> ALPQTVRIGTDTTYAPFSSKDAKGEFIGFAIDLGNEMCKRMQVKCTWVASDFDALIPSLKAKK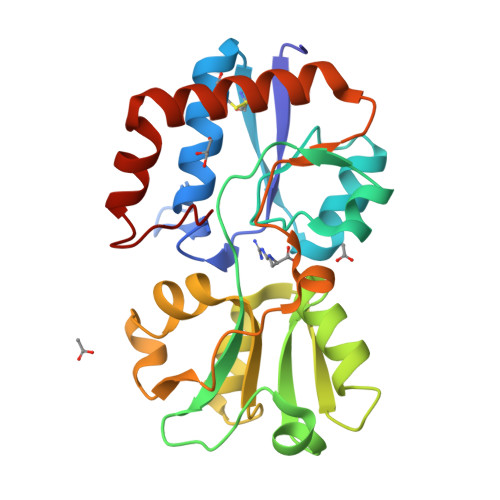IDAIISSLSITDKRQQEIAFSDKLYAADSRLIAAKGSPIQPTLESLKGKHVGVLQGSTQEAYANDNWRTKGVDVVAYANQDLIYSDLTAGRLDAALQDEVAASEGFLKQPAGKEYAFAGPSVKDKKYFGDGTGVGLRKDDTELKAAFDKALTELRQDGTYDKMAKKYFDFNVYGD Globulins are a class of storage proteins that belong to the most conserved and functionally diverse cupin superfamily. The pro-globulin consists of an acidic and a basic subunit bridged by a disulphide bond. 11S globulins predominantly exist as hexamers due to the non-covalent interactions between the trimers. In this study, we report the crystal structure of 11S homo-hexameric globulin complexed with Indole-3-acetic acid (IAA), an auxin, isolated from seeds of Wrightia tinctoria at 1.7 Å resolution.

It belongs to P212121 space group and has six monomers in an asymmetric unit forming two trimers. An asymmetric unit consists of six monomers arranged in hexameric assembly. These six monomers of WTG can be divided into two trimers (chains ABC and DEF); that are stacked together through hydrophobic and hydrogen-bonding interactions. The hydrophobic pocket formed at the interface of the tetramer (adjacent dimer from each trimer) on the IE surface sandwiched between two trimers act as the site for binding of the ligand. The indole ring snuggles into the cavity formed by proline residues of the acidic subunit of two monomers from opposite trimers, whereas the carboxyl group interacts with residues contributed by the basic subunit of two other monomers. The indole ring goes deep in the pocket and makes pi-sigma interaction with Pro121 of two chains lying diagonally opposite to each other. In one orientation, the amine group of the indole ring bonds with the backbone oxygen atom of Gly119 of chain E. The carboxyl side chain oxygen atom of auxin interacts with side chain NH2 and NE atoms of Arg427 of chain C and water molecules in the nearby vicinity. In all the chains, citrate interacts with backbone amino groups of Phe153, Ile295, Lys296, and the side-chain amine group of Arg294 through its carboxylic moiety. There was no density for any metal ion in all the three pockets. The results obtained from MALDI-MS and HRMS confirm the molecule associated with WTG is, indeed, indole −3 acetic acid. Results demonstrate a novel function of WTG in the storage of plant hormones that are essential for seed germination apart from its nutritional importance in seeds.

>MASTSFLQVLIALICLVLLCERSCLASRQSSPQSITEKQGIGECDLQRVNPLEPAHRIQHEAGYSEIWDPTSRELQCAGIDATRHVIENRGLFVPSYNNAPMLIIVVQGHGILGAVFPGCPETFQSFHPTEKEGGDSRGPDQTFRDQHQKVHFIRQGDVIALPAGIVHWAYNEATEKLVLLVIHDLSNRENQLDQNLRRYFLGGNQKGDEETWAVGSKNLLWNNVFQPLDPQFLGRASGVNSEIIKKLQSENDFRGYMVRVRDGLRLVRPSSEEPRPPRPLLDNGYEETLCTVRIKENLLNPERADIYTSRGGTVSTLNSYNLPILRKLQLSANREYLYPNAMIVPEWNNNAHSISYVTRGSGRLQVGGSSKSTVYDGDVRQGQLFIIPQNYVYLKQAGPQGLELYTVKTNDRAKATALVGRTSVIRAVPLDVWINVFQLTQDEARSLKYNREEITVLDPELPKPQPEGGGYYPWSIVA[6x]> GSDLTVSLIPVSGLKAGKNAPSAKIAKLVVNSTTLKEFGVRGISNNVVDSTGTAWRVAGKNTGKEIGVGLSSDSLRRSDSTEKWNGVNWMTFNSNDTLDIVLTGPAQNVTADTYPITLDVVGYQP;> VNQQLNSATKLFSVKLGATRVIYHAGTAGATLSVSNPQNYPILVQSSVKAADKSSPAPFLVMPPLFRLEANQQSQLRIVRTGGDMPTDRETLQWVCIKAVPPENEPSDTQAKGATLDLNLSINACDKL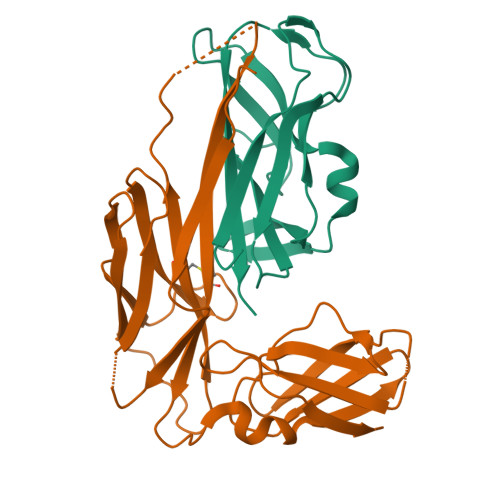IFRPDAVKGTPEDVAGNLRWVETGNKLKVENPTPFYMNLASVTVGGKPITGLEYVPPFADKTLNMPGSAHGDIEWRVITDFGGESHPFHYVLK>EQPEYKDKLIKLIKDGAISLGGGELIVRLNKRDMELIDDSTLWNLEKEVENATKKVTVLKKGEPVDIAGGCII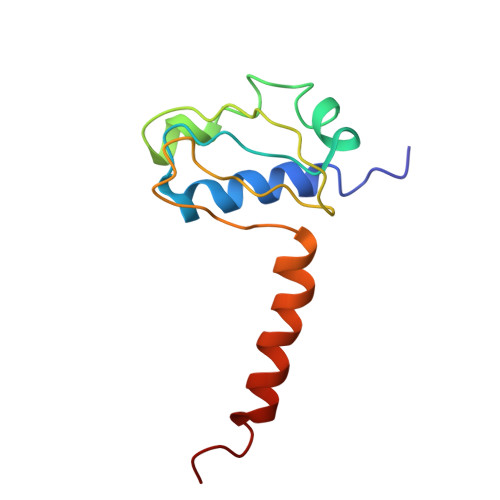ETADGLKSLDNSLEAIFNRNLNVIRARITEKLF[2x]>MSNLLTVHQNLPALPVDATSDEVRKNLMDMFRDRQAFSEHTWKMLLSVCRSWAAWCKLNNRKWFPAEPEDVRDYLLYLQARGLAVKTIQQHLGQLNMLHRRSGLPRPSDSNAVSLVMRRIRKENVDAGERAKQALAFERTDFDQVRSLMENSDRCQDIRNLAFLGIAYNTLLRIAEIARIRVKDISRTDGGRMLIHIGRTKTLVSTAGVEKALSLGVTKLVERWISVSGVADDPNNYLFCRVRKNGVAAPSATSQLSTRALEGIFEATHRLIYGAKDDSGQRYLAWSGHS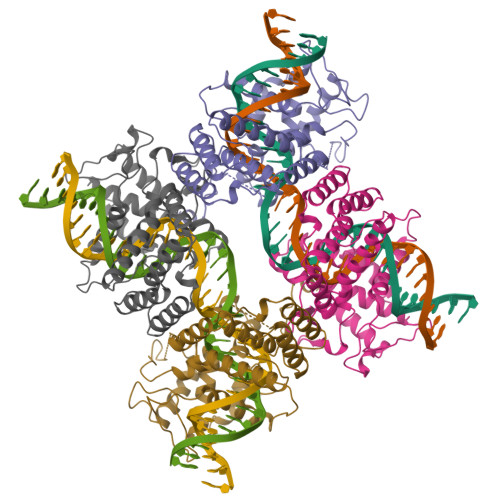ARVGAARDMARAGVSIPEIMQAGGWTNVNIVMNFIRNLDSETGAMVRLLEDGD[2x]> MCSHYQALKDQERMRKYFAAHPSAEVPADMWPRYMGAFIRRPLEWDSGDEAVPEREAATGRWGMIPPGTRPEKLAEASKKNTSNARSETAHQLWTFRNAWAKAQHC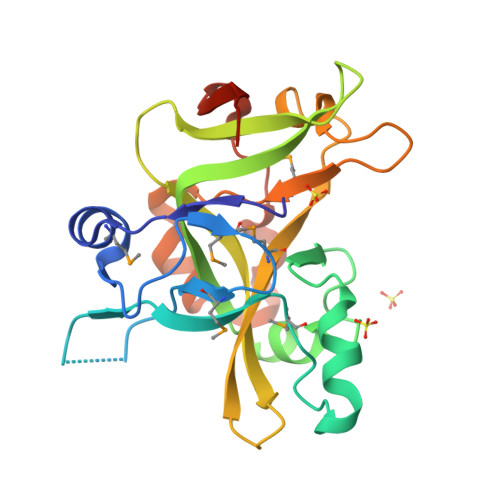IIPADAIYEPDWRSGKAVPTRFTRADGAPLGIAGLWDRYRNAAGEWIDSYTMLTINADDDPLFRDYHQAGKEKRMVVILPDGAYGDWLTAPATDTRDFLLPYPADRLVAAAVKLEHHHHHH>MGSSHHHHHHSSGLVPRGSMNQNLLVTKRDGSTERINLDKIHRVLDAAAEGLHNVSISQVELRSHIQFYDGIKTSDIHETIIKAAADLISRDAPDYQYLAARLAIFHLRKKAYGQFEPPALYDHVVKMVEMGKYDNHLLEDYTEEEFKQMDTFIDHDRDMTFSYAAVKQLEGKYLVQNRVTGEIYESAQFLYILVAACLFSNYPRETRLQYVKRFYDAVSTFKISLPTPIMSGVRTPTRQFSSCVLIECGDSLDSINATSSAIVKYVSQRAGIGINAGRIRALGSPIRGGEAFHTGCIPFYKHFQTAVKSCSQGGVRGGAATLFYPMWHLEVESLLVLKNNRGVEGNRVRHMDYGVQINKLMYTRLLKGEDITLFSPSDVPGLYDAFFADQEEFERLYTKYEKDDSIRKQRVKAVELFSLMMQERASTGRIYIQNVDHCNTHSPFDPAIAPVRQSNLCLEIALPTKPLNDVNDENGEIALCTLSAFNLGAINNLDELEELAILAVRALDALLDYQDYPIPAAKRGAMGRRTLGIGVINFAYYLAKHGKRYSDGSANNLTHKTFEAIQYYLLKASNELAKEQGACPWFNETTYAKGILPIDTYKKDLDTIANEPLHYDWEALRESIKTHGLRNSTLSALMPSETSSQISNATNGIEPPRGYVSIKASKDGILRQVVPDYEHLHDAYELLWEMPGNDGYLQLVGIMQKFIDQSISANTNYDPSRFPSGKVPMQQLLKDLLTAYKFGVKTLYYQNTRDGAEDAQDDLVPSIQDDGCESGACK[4x]

Class Ia ribonucleotide reductases (RNRs) are allosterically regulated by ATP and dATP to maintain the appropriate deoxyribonucleotide levels inside the cell for DNA biosynthesis and repair. The α2 subunit houses the active site and the allosteric sites, and the β2 subunit houses the di-iron-tyrosyl radical cofactor.3−6 On every round of turnover, these subunits come together to form an active α2β2 complex, which allows for the transfer of the radical species from β to α, affording ribonucleoside diphosphate reduction. Excess dATP inhibits RNR through the creation of an α–β interface that restricts the ability of β2 to obtain a position that is capable of radical transfer. ATP breaks the α–β interface, freeing β2 and restoring enzyme activity.

We reasoned that substitutions of either F87 or W28 with Ala would create room for ATP binding in site 2 regardless of the position of H59 and thus be independent of the presence of ATP in site 1. In other words, F87A and W28A substitutions would be expected to uncouple the binding of ATP to site 2 from the identity of the nucleotide effector in site 1. First, we wanted to determine if ATP could enter site 2 with dATP in site 1 in the W28A construct, so we grew crystals in the presence of a mixture of 3–5 mM ATP and 1 mM dATP. The resulting 3.40-Å resolution structure revealed clear density for two nucleotides in the activity site, but the identity of the site 1 nucleotide was ambiguous given the low resolution of the structure. Due to the lack of clarity about the identity of the nucleotide in site 1, this structure could not be used as evidence that a W28A substitution leads to site 1, 2 uncoupling. Unfortunately, attempts to obtain a high-resolution structure with ATP and dATP have so far been unsuccessful.> AMDKSAKAPVITIFDHRGCSRAPK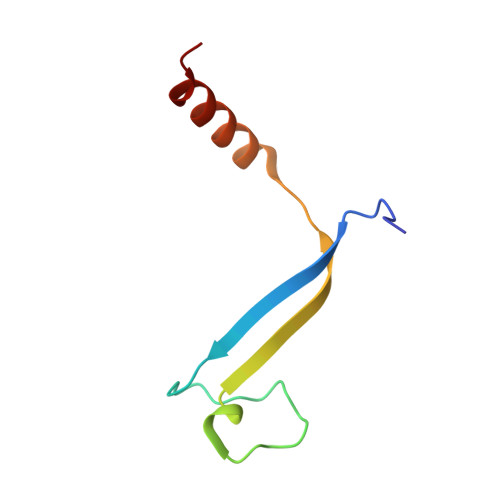EYTGAKAGGKDDEMMVKAQSVKIEVSTGTAEGVLATSLAKMTK> MATSRYEPVAEIGVGAYGTVYKARDPHSGHFVALKSVRVPNGEEGLPISTVREVALLRRLEAFEHPNVVRLMDVCATSRTDREIKVTLVFEHVDQDLRTYLDKAPPPGLPAETIKDLMRQFLRGLDFLHANCIVHRDLKPENILVTSGGTVKLADFGLARIYSYQMALDPVVVTLWYRAPEVLLQSTYATPVDMWSVGCIFAEMFRRKPLFCGNSEADQLGK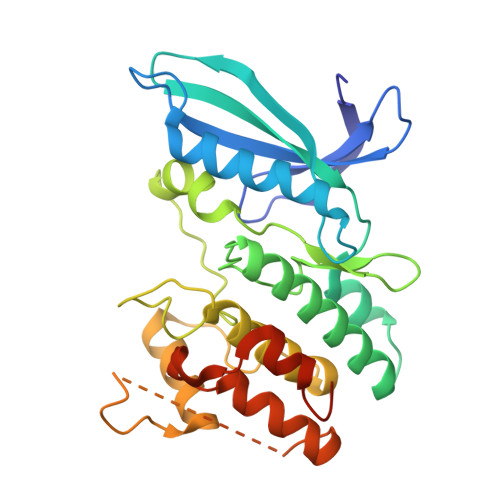IFDLIGLPPEDDWPRDVSLPRGAFPPRGPRPVQSVVPEMEESGAQLLLEMLTFNPHKRISAFRALQHSYLHKDEGNPEHHHHHH> MAHHHHH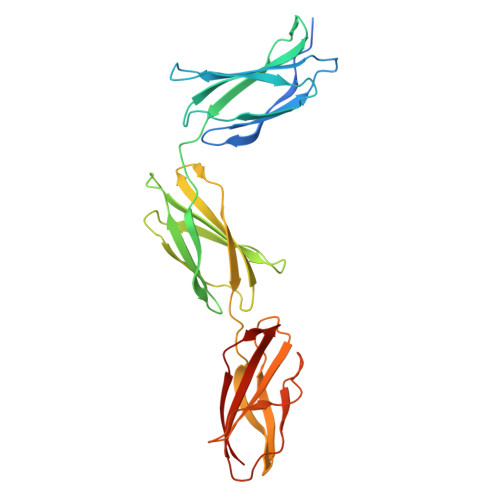HSSGLEVLFQGPAIPAPTDLKFTQVTPTSLSAQWTPPNVQLTGYRVRVTPKEKTGPMKEINLAPDSSSVVVSGLMVATKYEVSVYALKDTLTSRPAQGVVTTLENVSPPRRARVTDATETTITISWRTKTETITGFQVDAVPANGQTPIQRTIKPDVRSYTITGLQPGTDYKIYLYTLNDNARSSPVVIDASTAIDAPSNLRFLATTPNSLLVSWQPPRARITGYIIKYEKPGSPPREVVPRPRPGVTEATITGLEPGTEYTIYVIALKNNQKSEPLIGRKKT> PYF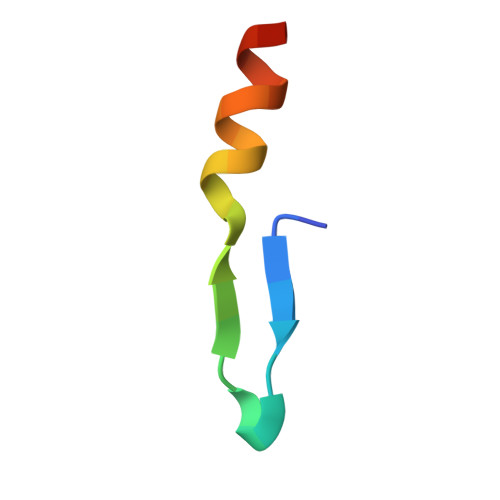VETPYGYQLDLDFLKYVDDIQKG Herein a bacterial pyranose oxidase from Oscillatoria princeps (OPOx) was biochemically characterized in detail. All-in-all, the results show that OPOx is a true pyranose-2-oxidase, resembling the fungal POxs. In contrast to the fungal pyranose oxidases, OPOx could be well expressed in Escherichia coli as soluble, fully flavinylated, and active oxidase. It was found to be highly thermostable (melting temperature >90 °C) and showed activity on glucose, exhibiting an exceptionally low KM value (48 μM). Elucidation of its crystal structure revealed similarities with fungal pyranose oxidases, such as being a tetramer with a large central void leading to a narrow substrate access tunnel.

In this study, a novel bacterial POx from O. princeps, dubbed OPOx was discovered, biochemically characterized and its structure was elucidated at a resolution of 2.6 Å. It marks the first reported bacterial POx crystal structure. According to the Pisa web server the interface area in the crystal structure between subunits A-B (C-D) is 4000 Å2, and A-D (B-C) is 785 Å2, while between A-C (B-D) it is 685 Å2 with a Complexation Significance Score (CSS) score of 0.63. In total, an area of 28,070 Å2 is buried upon tetramerization. OPOx’s monomeric subunit displays a typical GMC fold with a Rossmann fold flavin-binding domain and a substrate-binding domain. Similar to other POxs, the substantial central void directs to a narrow substrate channel that is regulated by a substrate loop, which is crystallized in the closed conformation and is hypothesized to rearrange to an (semi-)open state upon substrate proximity. For a productive binding mode the sugar must be oriented for oxidation at C2, the substrate-binding loop in the semi-open conformation and the side chain Oγ1 group of Thr127 is pointing away from the flavin N(5)/O(4) locus. However, in the determined OPOx structure the substrate-binding loop is closed and the Oγ1 group of Thr127 is pointing toward O4 and N5 of the FAD. His125-NE2 is indeed covalently bound to the 8α-methyl moiety of FAD as observed in the fungal enzymes. The FAD is further surrounded by hydrophobic residues and the catalytic residues His470 and Asn514 (the His-Asn pair). Inspection of the crystal structure revealed the presence of a salt-bridge forming glutamic acid (Glu69) near His125, which appears to push the histidine into a different conformation than observed in the bacterial POx-like oxidases that contain a non-covalent FAD.

>[4x]HHHHHHMSCKISAEVVIIGSGPVGATFARHLVENGKSVILVDAGPQRSPQPGEHLKNAYLYQKDRTNFSQIVNSELYKLSIPTSNVKLPNLDPSAYWAAGAVRNNMNPKQDPNTNMPYAQAAFAVGGMGIHWTCATPRLHPELERWHYITEWDELYAQAEKYFNTHTNVFERSLRGAAIKRRLEAHYNNQLDPNYPIQNLPVAAQRREDGEGEAFIHWTGPYDILKPVLTTEENLPNPNIRVLPNHIVQKLHHKGGKVEYAEVQSTEPWEKVEIYADIFIVAAAAIKTPQLLWNSQIRPKALGCYLSEHIMTFGQIVLSKEIVAEIKAEEKPYFKESPKMFHVAGNQKDPIDIPLYDPDPTLWIPVQKDRPWHCQIHKDNFSYGIVPDNIDDRLVVDLRWFGFVDQMPTNYVTFEEEIFDIHGMPQPTFHFQYPEQDAENAHRMMQDMTEVGLSIGGFLPTPEARPQFMAPGSSLHSMGTYRMGESDDGTSVVDAHSKVWGFDNLYLGGPGVIPKPNGANPTLTAAALAIRAANHILRN>GSSFSESALEKKLSELSNSQQSVQTLSLWLIHHRKHAGPIVSVWHRELRKAKSNRKLTFLYLANDVIQNSKRKGPEFTREFESVLVDAFSHVAREADEGCKKPLER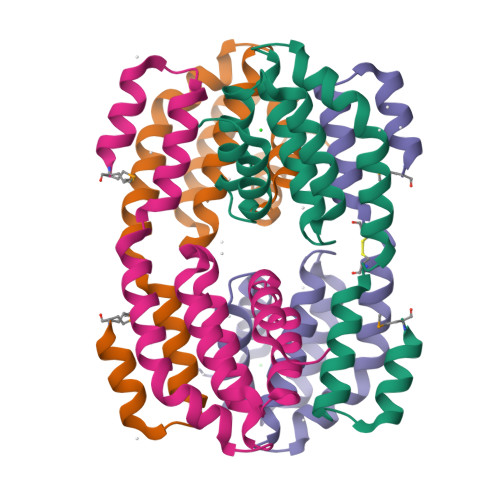LLNIWQERSVYGGEFIQQLKLSMEDSKSP[2x]>[2x]MFPDLKGKRVLITGSTEGIGLATARLFARAGAKVGLNSHVDPANIDETIASMRADGGDAAFFAADLATSEACQQLVDEFVAKFGGIDVLINNAGGLVGRKP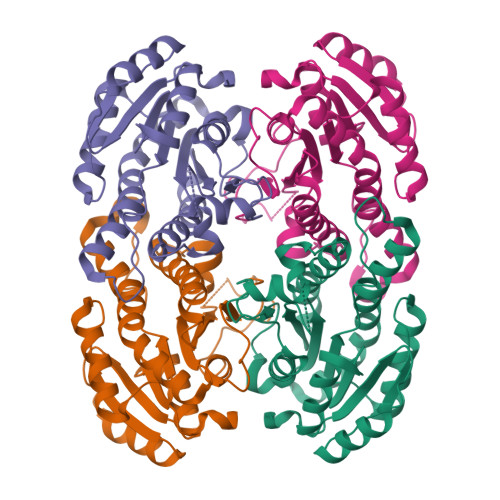LPEIDDTFYDAVMDANIRSVVMTTKFALPHLAAAAKASGQTSAVISTGSIAGHTGGGPGAGLYGAAKAFLHNVHKNWVDFHTKDGVRFNIVSPGTVDTAFHADKTQDVRDRISNGIPMGRFGTAEEMAPAFLFFASHLASGYITGQVLDINGGQYKH>[2x]GMTASSKRTKKQAILETALQLFVSQGFHGTSTATIAREAGVATGTLFHHFPSKEQLLEQLFLGVKQEFADAI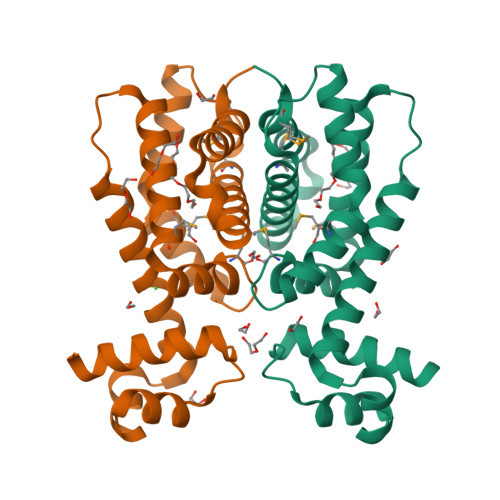QASVSSRGDLKQDAEQLWFAALTWAMANPLKQAFFQLYSMSPTVEQSVRDQAMHGILGFIAELIRQGQASGELAEYPIELMQDNCHGQYLAATRYFVDHPERWQQAHERSASFALFWNAMAVR1-[4-[[2-[(1-methylpyrazol-4-yl)amino]quinazolin-8-yl]amino]piperidin-1-yl]ethanone | 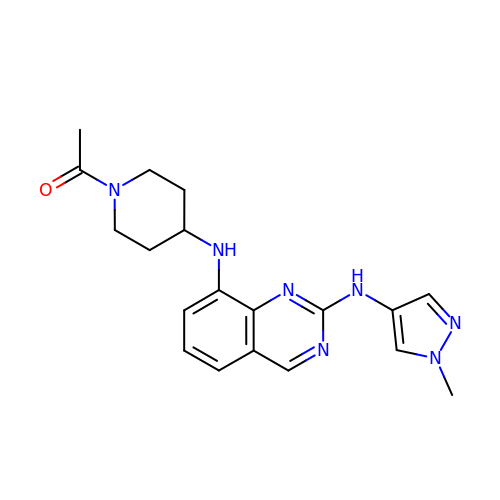C19 H23 N7 O | MYAXOPAVZLMPET-UHFFFAOYSA-N>MGSSHHHHHHSSGLVPRGSHMASMKSSNIYSPFDLKCEFTTNPLGVDKKNPIFSWKLRHLEKNEKQTAYQVIVSSSLETINDNIGDVWDTGKVLSSEQVIKYEGKELEPCKVYFWKVRWWDSKDQESPFSVVNTFETGLMNEENWKAKWITKKEHKYEVYSPDGAPFGLNYTIAYAPMFRKSFSISKKIKRARVYIAGLGLYELYINGERIGDRVLDPGQTDYKKRVLYTVYDVSKNIRDGKNAIGVILGNGRYVKEYGYDFPKLIIQVLVEYEDDSIEWIVSDESWKTTYGPITLNSLYHGEIYDGRKEIKGWNLPDFDDSTWENAILAEPPGGKLYSEIYPPIRITKTIKPIKMWSPEPGTYVYDFGQNYTGWIKIKVRTNESGKEIRIRHAELTYEDGTLNYSTNRTALATDVYITKGEGYEEYEPRFTYHGFRYVEILGYPGVPTLEDIEGKVVHTAVESNGEFICSNELINKIHHNIIWGQLSNLMSIPTDCPQRDERMGWMGDAQLSAEEAIFNFDMIGFYRKYLNDIRDAQKENGSLSDVIPPYWSIYPGDPAWSTAYITIAWYLYQYYGDKYVLEEHYEGFKKYVEFLKKLAPDYIVSFYKYGDWCQPGTVRPKDNSGELTSTFYFYHDVITLSKIAKLLGKEADYKYYSELADKIKSAFNKKFLKEKAYASIPTELSEENVKALLEKYPEDIKDFL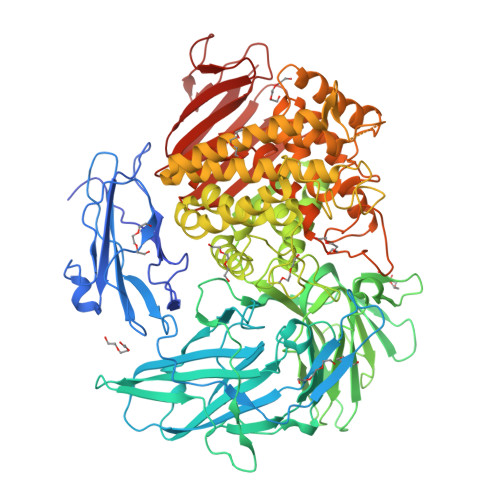RQQFTILSSLGMFTSQTLNTLPLYLNLVPEDKVQDVLKTLLEDIIIRHDYHLDTGIVATRYIFDVLTSYGYDEVAYKIVNQKTYPSFGYMIEEGATTLWERWEKLTSTGMNSHNHIMFGSVDAWFYRVIAGVRVGEPGWNKIIFEPHPVGDLKYAKARLNTIKGEVEINWQKTENIFSMRISVPVNSEGEVHVPKLFERFVVKEGDNIIYEKKGDLEENEKYIVIRVGSGSYNFYMEKI[2x]>[2x]DEKVVDEVKYSEEVCNEQVDL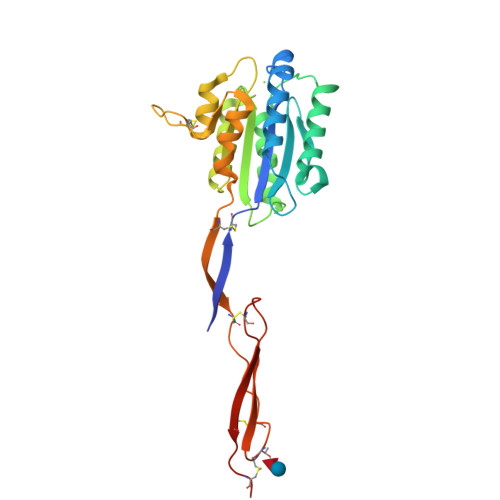YLLVDGSGSIGYPNWITKVIPMLNGLINSLSLSRDTINLYMNLFGSYTTELIRLGSGQSIDKRQALSKVTELRKTYTPYGTTSMTAALDEVQKHLNDRVNREKAIQLVILMTDGVPNSKYRALEVANKLKQRNVRLAVIGIGQGINHQFNRLIAGCRPREPNCKFYSYADWNEAVALIKPFIAKVCTEVERVANCGPWDPWTACSVTCGRGTHSRSRPSLHEKCTTHMVSECEEGECPHHHHHHA>[4x]YDPTKAGDIVKATKWPPKLPEIQDLAIRARVFIHKST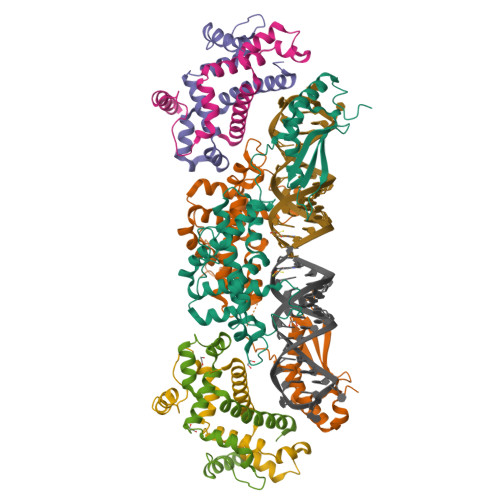IKDKVYLSGSEMINAHNERLEFLGDSILNSVMTLIIYNKFPDYSEGQLSTLRMNLVSNEQIKQWSIMYNFHEKLKTNFDLKDENSNFQNGKLKLYADVFEAYIGGLMEDDPRNNLPKIRKWLRKLAKPVIEEATRNQVALEKTDKLDMNAKRQLYSLIGYASLRLHYVTVKKPTAVDPNSIVECRVGDGTVLGTGVGRNIKIAGIRAAENALRDKKMLDFYAKQRAAIPRSESVLKDPS;>ISNYKYLEVIQLEHAVTKLVESYNKIIELSPNLVAYNEAVNNQDRVPVQILPSLSRYQLKLAAELKTLHDLKKDAILTEITDYENEFDTEQKQPILQEISKADMEKLEKLEQVKREKRE[8x]> MQLLSGIEQQQNNLLRAIEAQQHLLQLTVWGIKQLQARILAGGRGGHTTWM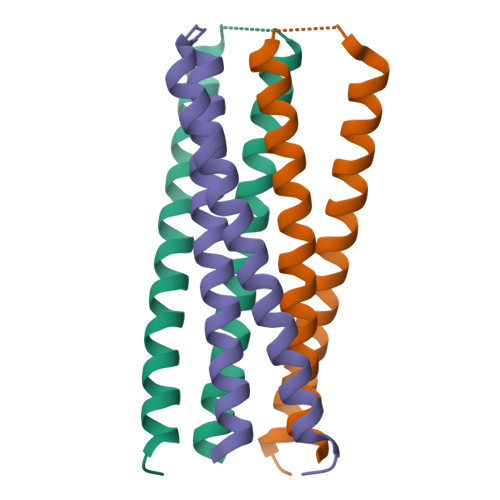EWDREINNYTSLIHSLIEESQNQQEKNEQELLGGHHHHHH>[4x]MIRSVVIVGGGTAGWMTASYLKAAFDDRIDVTLVESGNVRRIGVGEATFSTVRHFFDYLGLDEREWLPRCAGGYKLGIRFENWSEPGEYFYHPFERLRVVDGFNMAEWWLAVGDRRTSFSEACYLTHRLCEAKRAPRMLDGSLFASQVDESLGRSTLAEQRAQFPYAYHFDADEVARYLSEYAIARGVRHVVDDVQHVGQDERGWISGVHTKQHGEISGDLFVDCTGFRGLLINQTLGGRFQSFSDVLPNNRAVALRVPRENDEDMRPYTTATAMSAGWMWTIPLFKRDGNGYVYSDE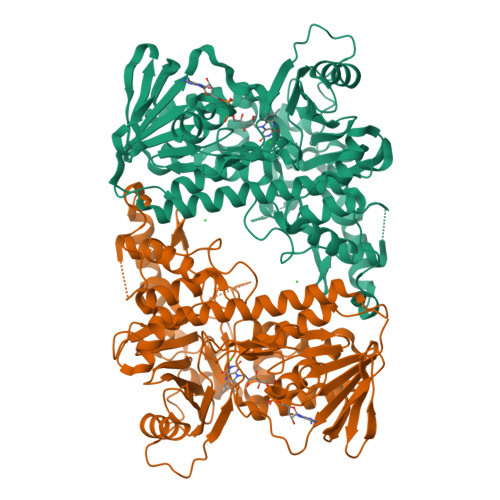FISPEEAERELRSTVAPGRDDLEANHIQMRIGRNERTWINNCVAVGLSAAFVEPLESTGIFFIQHAIEQLVKHFPGERWDPVLISAYNERMAHMVDGVKEFLVLHYKGAQREDTPYWKAAKTRAMPDGLARKLELSASHLLDEQTIYPYYHGFETYSWITMNLGLGIVPERPRPALLHMDPAPALAEFERLRREGDELIAALPSCYEYLASIQ>ASTLKSGSKEVENLKKPFMPPREVHVQVTHSMPPQKIEIFKSLDNWAEENILVHLKPVEKCWQPQDFLPDPASDGFDEQVRELRERAKEIPDDYFVVLVGDMITEEALPTYQTMLNTLDGVRDETGASPTSWAIWTRAWTAEENRHGDLLNKYLYLSGRVD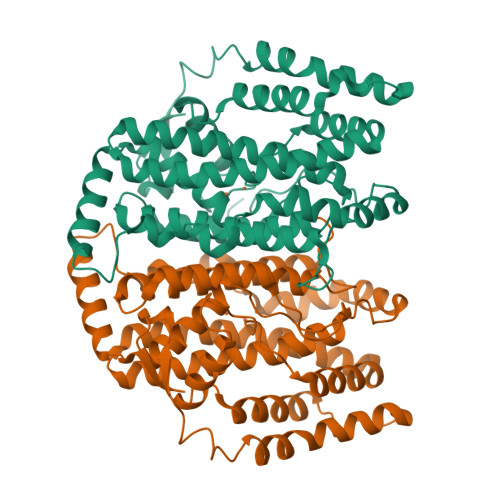MRQIEKTIQYLIGSGMDPRTENSPYLGFIYTSFQERADFISHGNTARQAKEHGDIKLAQICGTIAADEKRHETAYTKIVEKLFEIDPDGTVLAFADMMRKKISMPAHLMYDGRDDNLFDHFSAVAQRLGVYTAKDYADILEFLVGRWKVDKLTGLSAEGQKAQDYVCRLPPRIRRLEERAQGRAKEAPTMPFSWIFDRQVKL[6x]> HTLSTLAALPAAEIVRLANSQ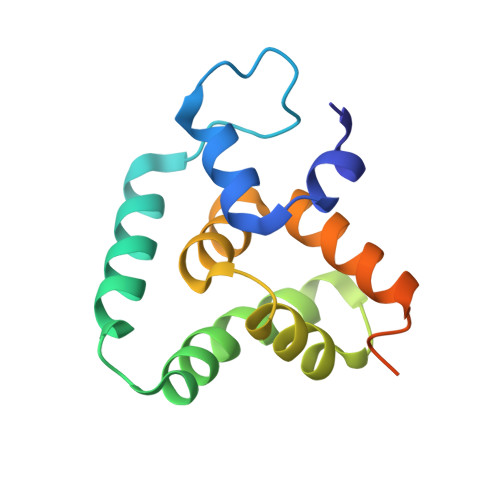SSSGLPLPKADPATVKATDDFIDSLQGKAAHDQKQKLGDQLFKKIRTFGVKGAPKLTIHLLDSEDLRALAHLMNSYEDVLKEKVQHKVAAGLNKVKGAPKLTIHLLDSEDLR>[8x]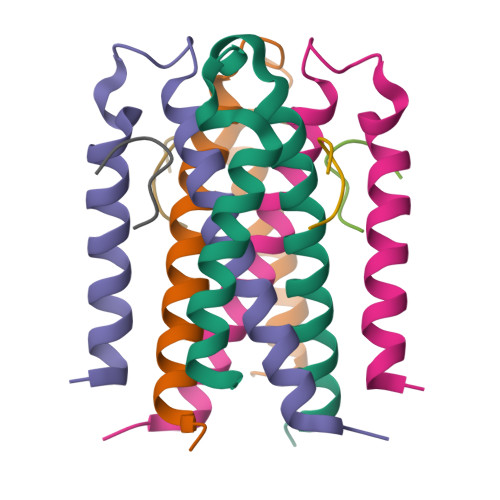ESAFNQTEFNKLLLECVVKTQSSVAKILGIESLSPHVSGNSKFEYANMVEDIREKVSSEMERFFPKNDDE;>GEDVEPGDDF[8x]> HGSMGDPVSRVSQCHAEGPENPKSAACRAAVAAGGTQALYDWNGIRIGNAAGKHQELIPDGRLCSANDPAFKGLDLARADWPATGVSSGSYTFKYRVTAPHKGTFKVYLTKPGYDPSKPLGWGDLDLSAPVATSTDPVASGGFYTFSGTLPERSGKHLLYAVWQRSDSPEAFYSCSDVTFG

Bacterial lytic polysaccharide monooxygenases (LPMOs) are known to oxidize the most abundant and recalcitrant polymers in Nature, namely cellulose and chitin. The genome of the model actinomycete Streptomyces coelicolor A3(2) encodes seven putative LPMOs, of which, upon phylogenetic analysis, four group with typical chitin-oxidizing LPMOs, two with typical cellulose-active LPMOs, and one which stands out by being part of a subclade of non-characterized enzymes. The latter enzyme, called ScLPMO10D, and most of the enzymes found in this subclade are unique, not only because of variation in the catalytic domain, but also as their C-terminus contains a cell wall sorting signal (CWSS), which flags the LPMO for covalent anchoring to the cell wall. While showing several structural and functional features typical for bacterial cellulose active LPMOs, ScLPMO10D is only active on chitin.

The structure of the catalytic domain of ScLPMO10D (residues 34–214, lacking the linker and the CWSS), hereafter called ScLPMO10DCD, was determined to 1.37 Å resolution with a single molecule in the asymmetric unit using the crystal structure of LPMO10A from Tectaria macrodonta (Tma12; PDB ID: 6IF738) as the starting model. The structure shows the typical LPMO fold with a central β-sandwich built up by two distorted β-sheets that are connected by several loops and helices. The active site of ScLPMO10D is formed by His34 and His134, which coordinate the bound copper cofactor in a T-shaped geometry. No water molecules were found adjacent to the copper, which indicates that the copper had been photo-reduced during data collection. The residues in the secondary coordination sphere resemble those found in C1-oxidizing cellulose-active AA10 LPMOs, such as ScLPMO10C26 and in the atypical chitin-active CjLPMO10A44. In ScLPMO10D, an additional arginine (Arg79) is interacting with Glu203 that together with Arg198 forms a remarkable arrangement that has, to the best of our knowledge, not been observed in any other LPMO. Generally, it is worth noting the considerable variation in second sphere residues, the functional implications of which are largely unknown. It is also worth noting that the arrangement of a catalytically crucial glutamate (Glu203) interacting closely with two positively charged residues (Arg79 and Arg198) really stands out from the active site arrangements found in other LPMOs. Like CjLPMO10A44, ScLPMO10D shows a “hybrid”-type catalytic center with features known from both cellulose-active and chitin-active LPMO10s. While Arg198 and Glu203 in ScLPMO10D are common to cellulose-active LPMO10s, Asn76 and Thr131 are common to chitin-active LPMOs.Kinesins are microtubule-based molecular motors that drive long-range intracellular transport or organize intricate microtubule networks. When not transporting cargoes, processive kinesin motors (kinesin-1 to -3) often adopt an autoinhibited conformation to avoid the futile consumption of ATP and the potential blockage of microtubule tracks. Instead of forming a constitutive dimer, most of kinesin-3 motors primarily exist as a self-folded monomer for autoinhibition, although some kinesin-3 members can adopt an autoinhibited dimeric conformation. In addition to the N-terminal motor domain (MD) and neck domain (containing the neck linker (NL) and neck coil (NC)), kinesin-3 contains a family-specific forkhead-associated (FHA) domain sandwiched by two coiled-coil segments (coiled-coil 1 (CC1) and CC2) and a characteristic membrane-associated guanylate kinase homolog (MAGUK)-binding stalk (MBS) domain in the middle.

In this study, we determine the full-length structure of the kinesin-3 motor KLP-6 (kinesin-like protein 6 in Caenorhabditis elegans for intraflagellar transport in cilia and mitochondrial transport in neurons) in a compact self-folded state. The structure was determined by the molecular replacement method (using the structures of the MD and the FHA and MBS domains of KIF13B as the searching models) and refined to 3.2 Å. In the structure of KLP-6, the extreme N-terminus, a stretch of the C-terminal tail and several internal loops could not be resolved due to their poor electron density maps, and the structure comprises residues from 5 to 842 with the missing of several flexible loops (as indicated by dashed lines in Fig. 1c). In contrast, none of the coiled-coil segments form a canonical coiled-coil dimer, but instead the NC and CC2 adopt a single helical structure and CC1 is melted into three short helices (CC1a to CC1c). Unexpectedly, from the overall view of the structure, all the coiled-coil segments and domains of KLP-6 fold back to successively wrap around the MD to form a self-folded compact monomer, consistent with the monomeric state in solution. Finally, in this compact structure, the NL is docked onto the MD, and ADP and Mg2+ are in the nucleotide-binding pocket of the MD (based on their well-resolved electron density maps). CC1 is melted into several short helices that associate with the NC and MD to inhibit the entire neck domain, while CC2 binds to both the FHA and MBS domains and integrates with the newly identified MATH domain in the tail region to form a supramodule. In addition to contacting with Switch I of the MD, the signature residue D458 from this β1-β2 loop (referred to as the D-loop) makes the electrostatic interactions with Mg2+, together with the phosphate group of ADP and a serine from the P-loop of the MD, to stably chelate this ion in the nucleotide-binding pocket.

>[2x]MGKGDSIIVAVRVRPFNDREKTRNCKLVIEMPDEETTVIRDPKTNDEKRFTYDHSYWSHDGFSEKKNGYLEPTDPHYADQRRVFEDLGRGVLANAWAGYNCSLFAYGQTGSGKSYSIVGFKNNKGIVPIVCEELFKQIADNKKKNMQFEVFVSMMEIYCEKVRDLLSSTPPPKGGLKVREHPKNGFYVENLTTVPVNSFKEIEAKIEEGTKSRTIAATQMNATSSRAHTIVKITFNQKSSKQAGGTSMKKSEINLVDLAGSERQSAAGTEGDRLKEGIVINQSLTTLGRVIKALHDSQKAKSGKKTQIPYRDSVLTCLLKNALGGNSKTIMIAAISPADINFEETLSTLRFADRAKSIKTNAVVNENQTERALRELREENLRLQSQIQGGTAGDASNEEIEKLRRQLAENQKEMEEMEKSWQQKIAEEAAKHASGASEKVEMEAKKKKMCHLWNLNEDPALTNVIVHFIPVGESVVGNKPTSSGNFIQMSGLSILPQHVTLKNDGNNQIHLSPCSEDLDIFINGKPVHGETQLQQNDRVFFGGNHLYVFNNPTKKGIRTDITYENAQAEIAQNHAAALGNRGLGGGSKRDLILEEELMSTLPLVQRANAMATELGRNVKFEIVLVSPEMRGLTSGLTEIWVKVHNISEDTYFLWEKSRFMNRYYGMQEMYEAKQDGSEDWNMPKERDPFYEPPDSPVFIASSVVFLQSLAYLIDVEEQFPIVDLSGQEIGLLTVGLSPCSTTGKELRGEYVEDPDQLIGKNIAFKVKVISAVGLPRRILKSNCKYRFFGSKKMTTTATVSGNTPAYGHEETFQFKPVTKEVADYLANSNLYITFWGTQRPRGASSRKNSISTIGSNEAREGPNKAKRVERLVHQAKTSENRNISVKALETVLKGVDDNENRKTRKQSMKKAGSTTIKSRSGSKKPKAKGTKLLEVLFQGPHHHHHHGSGSGSWSHPQFEK2-[(4,6-dimethylpyrimidin-2-yl)sulfanyl]-N-[5-(naphthalen-1-ylmethyl)-1,3-thiazol-2-yl]acetamide 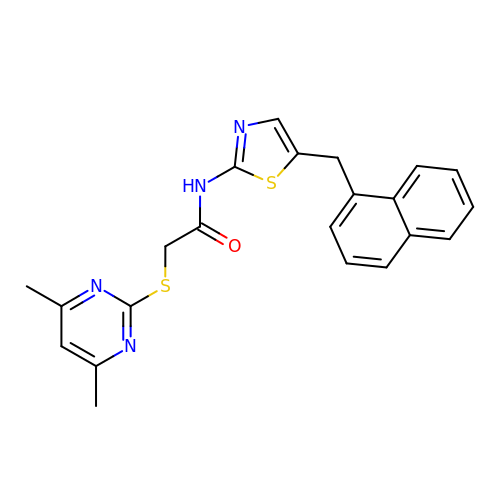| C22 H20 N4 O S2 | MENNDDDTIIZDDN-UHFFFAOYSA-N> ICQSTSNHLWLLSDILGQGATANVFRGRHKKTGDLYAVKVFNNISFLRPVDVQMREFEVLKKLNHKNIVKLFAIEEETTTRHKVLIMEFCPCGSLYTVLEEPSNAYGLPESEFLIVLRDVVGGMNHLRENGIVHRDIKPGNIMRVIGEDGQSVYKLTDFGAARELEDDEQFVSLYGTEEYLHPDMYERAVLRKDHQKKYGATVDLWSVGVTFYHAATGSLPFRPFEGPRRNKEVMYKIITGKPSGAISGVQKAENGPIDWSGDMPLSCSLSQGLQALLTPVLANILEADQEKCWGFDQFFAETSDVLHRMVIHVFSLQHMTAHKIYIHSYNTAAVFHELVYKQTKIVSSNQELIYEGRRLVLELGRLAQHFPKTTEENPIFVTSREQLNTVGLRYEKISLPKIHPRYDLDGDASMAKAVTGVVCYACRTASTLLLYQELMRKGVRWLVELVKDDYNETVHKKTEVVITLDFCIRNIEKTVKVYE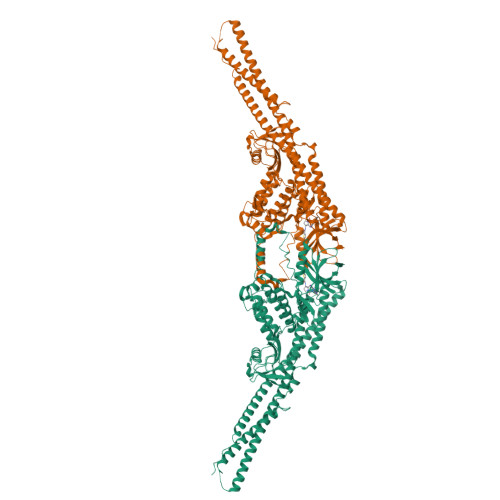KLMKVNLEAAELGEISDIHTKLLRLSSSQGTIESSLQDISSRLSPGGLLADTWAHQEGTHPRDRNVEKLQVLLNCITEIYYQFKKDKAERRLAYNEEQIHKFDKQKLYYHATKAMSHFSEECVRKYEAFKDKSEEWMRKMLHLRKQLLSLTNQCFDIEEEVSKYQDYTNELQE> GHFSVLLDVKHFSPEEIAVKVVGEHVEVHARHEERPDEHGFVAREFHRRYRL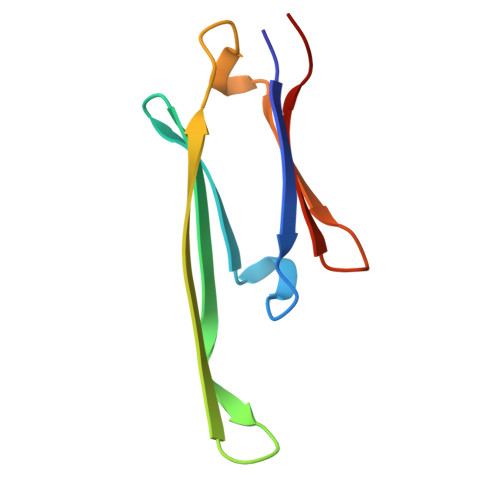PPGVDPAAVTSALSPEGVLSIQAAPA>MPAKLGYWKIRGLQQPVRLLLEYLGEEYEEHLYGRDDREKWLGDKFNMGLDLPNLPYYIDDKCKLTQSVAIMRYIADKHGMLGSTPEERARISMIEGAAMDLRMGFVRVCYNPKFEEVKGDYLKELPTTLKMWSNFLGDRHYLTGSSVSHVDFMVYEALD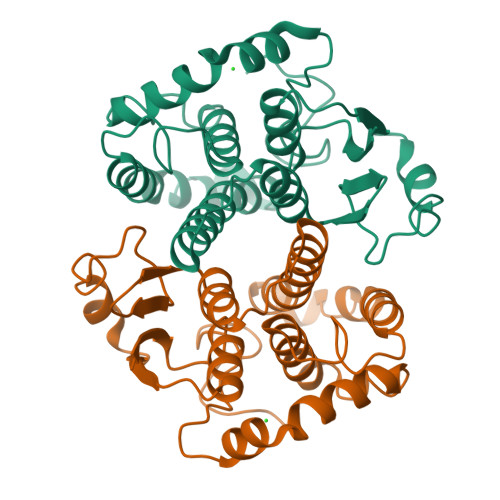CIRYLAPQCLEDFPKLKEFKSRIEDLPKIKAYMESEKFIKWPLNSWIASFGGGDAAPA[12x]>MSKAGASLATCYGPVSADVMAKAENIRLLILDVDGVLSDGLIYMGNNGEELKAFNVRDGYGIRCALTSDIEVAIITGRKAKLVEDRCATLGITHLYQGQSNKLIAFSDLLEKLAIAPENVAYVGD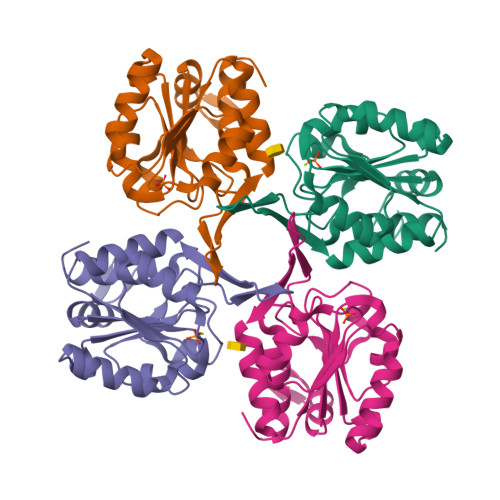DLIDWPVMEKVGLSVAVADAHPLLIPRADYVTRIAGGRGAVREVCDLLLLAQGKL[4x]> MRPVVSTGKAWCCTVLSAFGVVILSVIAHLFNTNHESFVGSINDPEDGPAVAHTVYLAAL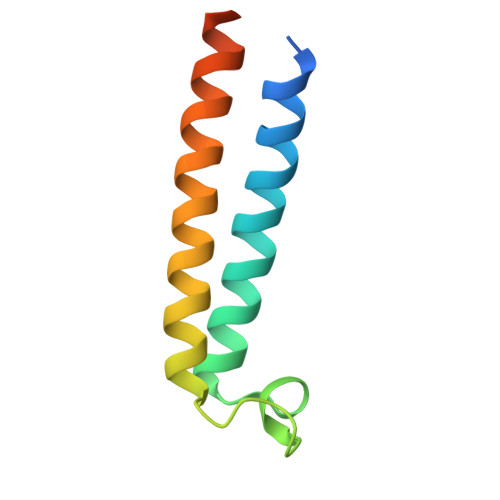VYLVFFVFCGFQVYLARRKPSIELR>MRCIGMSNRDFVEGVSGGSWVDIVLEHGSCVTTMAKNKPTLDFELIKTEAKQPATLRKYCIEAKLTNTTTESRCPTQGEPSLNEEQDKRFVCKHSMVDRGWGNGCGLFGKGGIVTCAMFRCKKNMEGKVVQPENLEYTIVITPHSGEEHAVGNDTGKHGKEIKITPQSSITEAELTGYGTVTMECSPRTGLDFNEMVLLQMENKAWLVHRQWFLDLPLPWLPGADTQGSNWIQKETLVTFKNPHAKKQDVVVLGSQEGAMHTALTGATEIQMSSGNLLFTGHLKCRLRMDKLQLKGM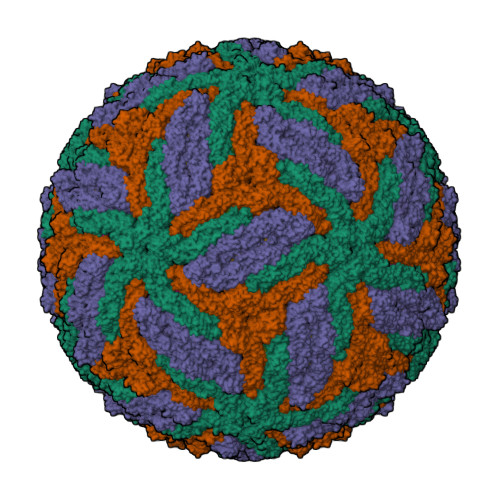SYSMCTGKFKVVKEIAETQHGTIVIRVQYEGDGSPCKIPFEIMDLEKRHVLGRLITVNPIVTEKDSPVNIEAEPPFGDSYIIIGVEPGQLKLNWFKKGSSIGQMFETTMRGAKRMAILGDTAWDFGSLGGVFTSIGKALHQVFGAIYGAAFSGVSWTMKILIGVIITWIGMNSRSTSLSVTLVLVGIVTLYLGVMVQA[3x];>SVALVPHVGMGLETRTETWMSSEGAWKHVQRIETWILRHPGFTMMAAILAYTIGTTHFQRALIFILLTAVTPSMT[3x]>GSDVVDPDIFNRDPRDHYDLLQRLGGGTYGEVFKARDKVSGDLVALKMVKMEPDDDVSTLQKEILILKTCRHANIVAYHGSYLWLQKLWICMEFCGAGSLQDIYQVTGSLSELQ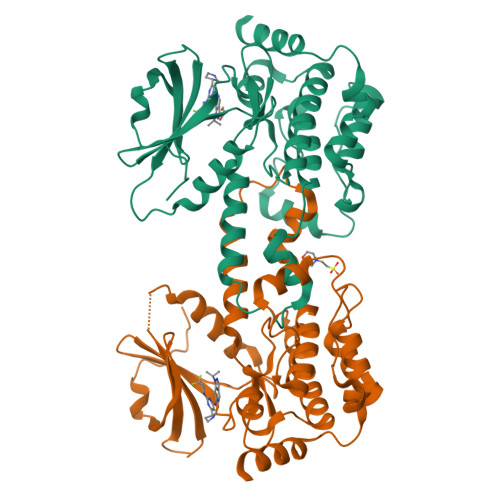ISYVCREVLQGLAYLHSQKKIHRDIKGANILINDAGEVRLADFGISAQIGAELARRLEFIGTPYWMAPEVAAVALKGGYNELCDIWSLGITAIELAELQPPLFDVHPLRVLFLMTKSGYQPPRLKEKGKWSAAFHNFIKVTLTKSPKKRPSATKMLSHQLVSQPGLNRGLILDLLDKLKNGNS[2x]>MGGGPNTGRDKDHLLKYNVGDLVWSKVSGYPWWPCMVSADPLLHSYTKLKGQKKSARQYHVQFFGDAPERAWIFEKSLVAFEGEGQFEKLCQESAKQAPTKAEKIKLLKPISGKLRAQWEMGIVQAE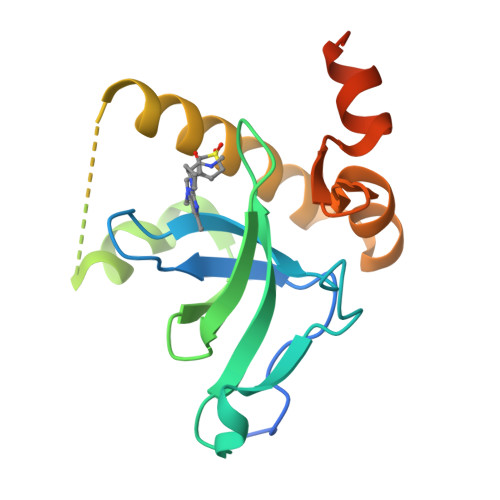EAASMSVEERKAKFTFLYVGDQLHLNPQVAKEAGIAAEGGGENLYFQGS[2x]> SMPAKSPVIVDLKFIPEEVEAALAGAFPGREVIDLADP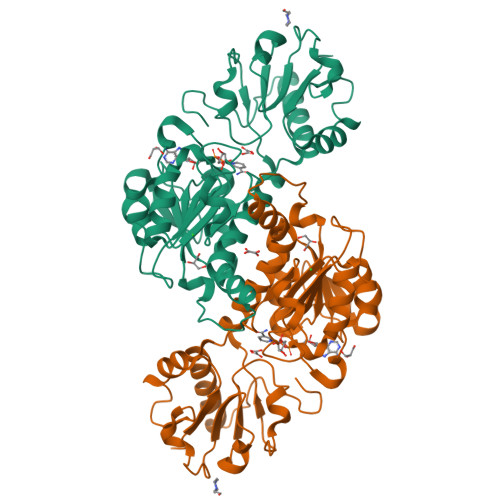AHQERDLSGIDYAVVWKSAPDLFSRAPDLKVVFSGGAGVDHVLTLPGLPDVPLVRFVDRTLTTRMSEWVMMQCLLHLRQHRAYEALAKKHEWRDLSQPEAADVTVGIMGMGVLGQDAARKLAAMGFKVIGWSRSKRVIEGVETYDAAGLDAFLGRTDFLVGLLPLTPDTRGIFNAALFAKLSRNGPFGAPVFINAGRGGSQVEADILECLDSGVLGGASLDVFEREPLSPESRFWDMPNVYVTPHVAASSDVRALFVHVEHQIARFESGLPLEHVVDKVAGY>LDCTVIDGNLKQIDAGSGSVVGVNNLNETFVLIDNVFTKISGSLKHFSVGPAGQLGVNTANNIFKYQSGGFVQLAGLLKQVDAGGDQIIAGVNMYDDIYCLNMDANNKWPSSNTPWVQLNGKLKYYSCGPYSCWGVNSNDQIFIMKDVSSNVCSGSGSF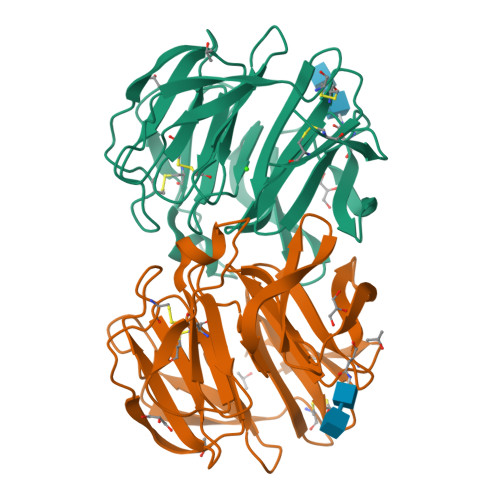INIPGLLSMIEVATDGSVFGVNSQGNLYQRTGVTRSKPDGTDWISMVACPNGHKHVSFDLGVLWLVCVDGSIRKCILTD[2x]> MENTENSVASKSIKNLEPKIIH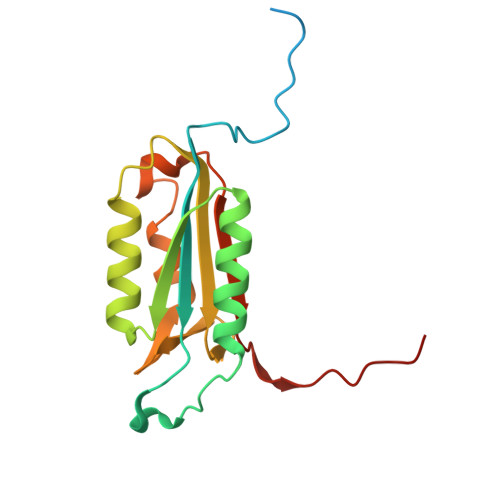GSESMASGISLDNSYKMDYPEMGLCIIINNKNFHKSTGMTSRSGTDVDAANLRETFRNLKYEVRNKNDLTREEIVELMRDVSKEDHSKRSSFVCVLLSHGEEGIIFGTNGPVDLKKITNFFRGDRCRELTGKPKLFIIQACRGTELDCGIETD7-(N-(10-hydroxydecanoyl)-aminopentenyl)-7-deaza-2'-dATP 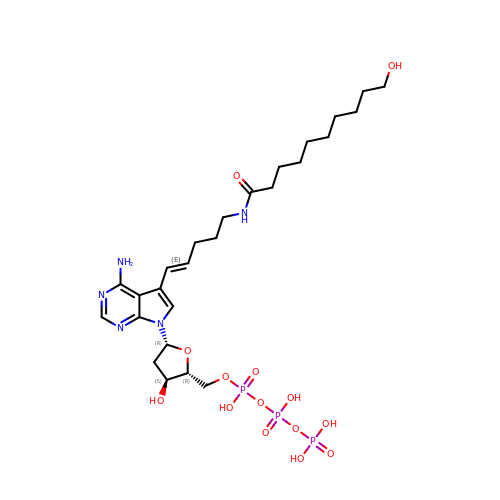| C26 H44 N5 O14 P3 | KGSINQKQGHRQNT-MNMHHJAXSA-N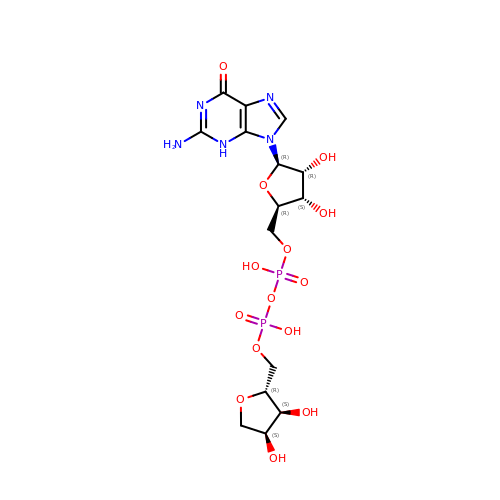GUANOSINE DIPHOSPHATE RIBOSE | C15 H23 N5 O14 P2 | NOLLEWZDVQOFJY-ZVIMGNLFSA-N>[5x]EAEAADRADILYNIRQTSRPDVIPTQRDRPVAVSVSLKFINILEVNEITNEVDVVFWQQTTWSDRTLAWNSSHSPDQVSVPISSLWVPDLAAYNAISKPEVLTPQLARVVSDGEVLYM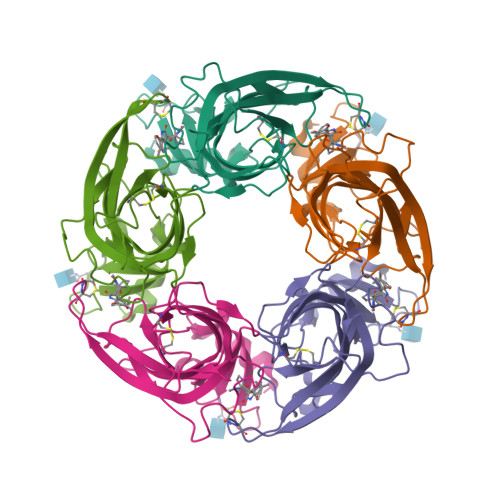PSIRQRFSCDVSGVDTESGATCRIKIGSWTHHSREISVDPTTENSDDSEYFSQYSRFEILDVTQKKNSVTYSCCPEAYEDVEVSLNFRKKGRSEIL>[4x]MVKSKIYIDKIYWERVQLFVEGHSENLDLEDSNFVLRNLTETRTMKANDVKIDGNQFVCRFNVAILDNGYYLPEDKYLLVNEQELDYIAQLNPDV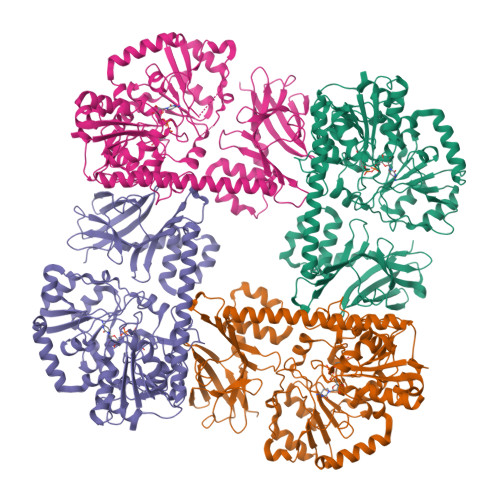INDAYQNLKPEQEEEYNELETQNGKINFLLQTYLKEFRKGGISKKTVYTVTPEISSDVNEFVLDVVVTTPEVKSIYIVRKYKELRKYFRKQSFNTRQFIFKAIFNTTKFFHLKKGNTVLFTSDSRPTMSGNFEYIYNEMLRQNLDKKYDIHTVFKANITDRRGIIDKFRLPYLLGKADYIFVDDFHPLIYTVRFRRSQEVIQVWNAVGAFKTVGFSRTGKKGGPFIDSLNHRSYTKAYVSSETDIPFYAEAFGIKEKNVVPTGVPRTDVLFDEAYATQIKQEMEDELPIIKGKKVILFAPTFRGSGHGTAHYPFFKIDFERLARYCEKNNAVVLFKMHPFVKNRLNIADKHKQYFVDVSDFREVNDILFITDLLISDYSSLIYEYAVFKKPMIFYAFDLEDYITTRDFYEPYESFVPGKIVQSFDALMDALDNEDYEGEKVIPFLDKHFKYQDGRSSERLVRNLFGSKLVPRGSAAAALEHHHHHHHH> GTVSDTNEKPKEEIKIVEPNGAEKTKLNLNFGVGKLNISGNEEKLMKGKFIYSENEWKPEIKYEVKDKDGELEISQPGLKSGNVSLNNKRNEWN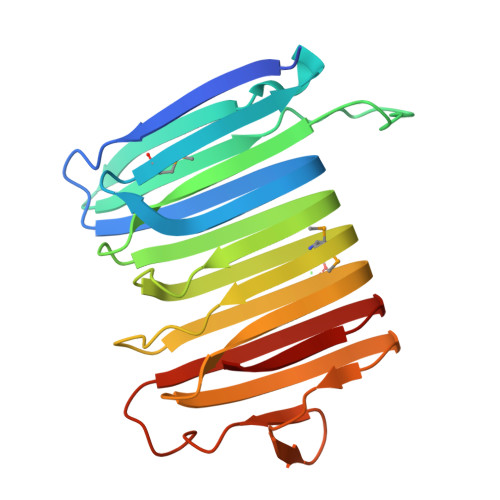INLNEKIPTEIKLSLGTGEFKADLSKINLKELNVGMGVGKVDLDISGNYKNNVKVNIEGGVGEATVYLPKSIGVKIKAEKGVGAVNANGFIVEGENIYKNSQYGKSKNSIEVNIEAGVGAINIKQK> MARQNLKSTDRAVQQMLDKAKREGIQTVWDRYEAMKPQCGFGETGLCCRHCLQGPCRINPFGDEPKVGICGATAEVIVARGLDRSIAAGAAGHSGHAKHLAHTLKKAVQGKAASYMIKDRTKLHSIAKRLGIPTEGQKDEDIALEVAKAALADFHEKDTPVLWVTTVLPPSRVKVLSAHGLIPAGIDHEIAEIMHRTSMGCDADAQNLLLGGLRCSLADLAGCYMGTDLADILFGTPAPVVTESNLGVLKADAVNVAVHGHNPVLSDIIVSVSKEMENEARAAGATGINVVGICCTGNEVLMRHGIPACTHSVSQEMAM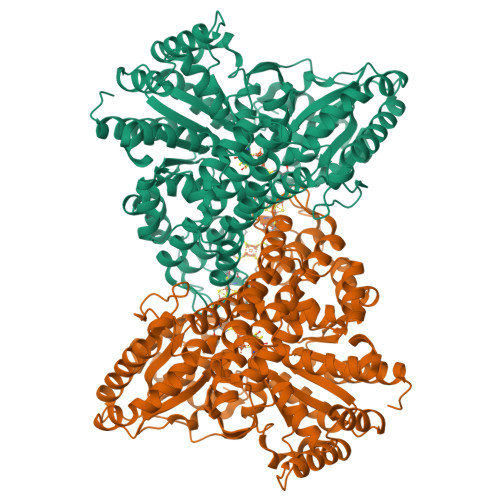ITGALDAMILDYQCIQPSVATIAECTGTTVITTMEMSKITGATHVNFAEEAAVENAKQILRLAIDTFKRRKGKPVEIPNIKTKVVAGFSTEAIINALSKLNANDPLKPLIDNVVNGNIRGVCLFAGCNNVKVPQDQNFTTIARKLLKQNVLVVATGCGAGALMRHGFMDPANVDELCGDGLKAVLTAIGEANGLGGPLPPVLHMGSCVDNSRAVALVAALANRLGVDLDRLPVVASAAEAMHEKAVATGTWAVTIGLPTHIGVLPPITGSLPVTQILTSSVKDITGGYFIVELDPETAADKLLAAINERRAGLGLPW> AQMTMVQAITDALRIELKNDPNVLIFGEDVGVNGGVFRATEGLQAEFGEDRVFDTPLAESGIGGLAIGLALQGFRPVPEIQFFGFVYEVMDSICGQMARIRYRTGGRYHMPITIRSPFGGGVHTPELHSDSLEGLVAQQPGLKVVIPSTPYDAKGLLISAIRDNDPVIFLEHLKLYRSFRQEVPEGEYTIPIGKADIKREGKDITIIAYGAMV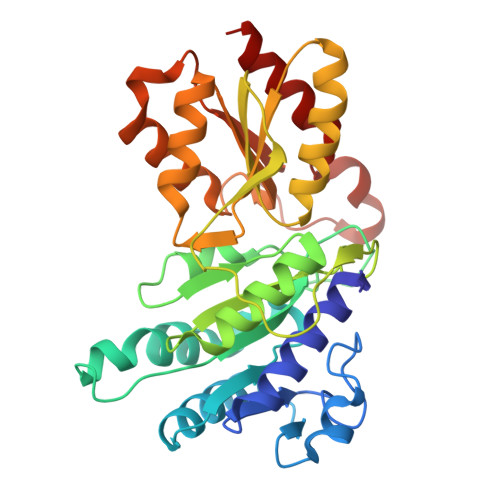HESLKAAAELEKEGISAEVVDLRTVQPLDIETIIGSVEKTGRAIVVQEAQRQAGIAANVVAEINERAILSLEAPVLRVAAPDTVYPFAQAESVWLPNFKDVIETAKKVMNF> MKRNHYLFTLILLLGCSIFVKASDTVFVHQTQIPILIERQDNVLFYFRLDAKESRMMDEIVLDFGKSVNLSDVQAVKLYYGGTEALQDKGKKRFAPVDYISSHRPGNTLAAIP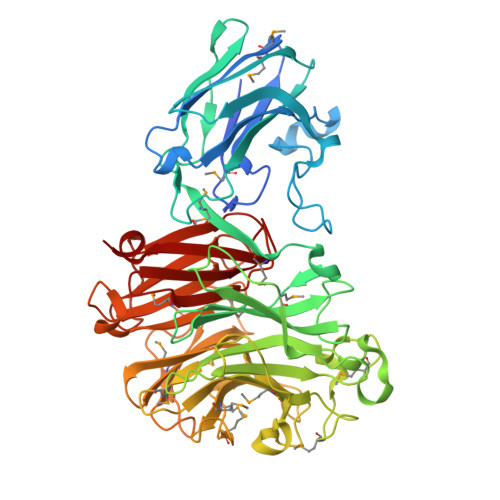SYSIKCAEALQPSAKVVLKSHYKLFPGINFFWISLQMKPETSLFTKISSELQSVKIDGKEAICEERSPKDIIHRMAVGVRHAGDDGSASFRIPGLVTSNKGTLLGVYDVRYNSSVDLQEYVDVGLSRSTDGGKTWEKMRLPLSFGEYDGLPAAQNGVGDPSILVDTQTNTIWVVAAWTHGMGNQRAWWSSHPGMDLYQTAQLVMAKSTDDGKTWSKPINITEQVKDPSWYFLLQGPGRGITMSDGTLVFPTQFIDSTRVPNAGIMYSKDRGKTWKMHNMARTNTTEAQVVETEPGVLMLNMRDNRGGSRAVAITKDLGKTWTEHPSSRKALQEPVCMASLIHVEAEDNVLDKDILLFSNPNTTRGRNHITIKASLDDGLTWLPEHQLMLDEGEGWGYSCLTMIDRETIGILYESSAAHMTFQAVKLKDLIR>[4x]MKVAPAPASGQPGGGSKKPSDYGCQLHYKHARVVEPESTTDDGMKRLKDVGDKGTLITAAELGLVDKYRDLKRAGQDILTCDWPYHYSSILYACYGNQYKILQMVEREFVGSTQELTAMHTTRCWVGKNSAMVAAYQGHLETMLYIIDLDMQGKFTEDLFKQRDVMGKNAMMWAASQGHTDTIEVLLVRSLYRLLPEDCADPLVLKTRWKLVSLLADLASHCRDYDPGCSRSFFQEVLASIKYDPVEGARQEEAAAAGGGGSAREGAALHEPTWGVDDGEEEERRHGVKHSDLVGKSAASTTAAAAAGGKTASGKPGEPGGGGAVKLKDVHITVRTLQGVIVSAYRAGMNCMGVIMYCQSLLQQARYFDDLVAQLTAWEVKLLDTCRNKQEVQAILAPTEDDPSEPVGYALATFDKAFLSHKFVQQIFTEKWDTMGVTDYTKSLFGVVWGGCSLVVAFAAWATICPLVVVARSFLSPVQDFMMRGKVIVDSRFPWHVPLYRWLLTQCALITFTVLLSYLVFSFDPSDPVPASVAPLNTFLAVWCAAILVDEVQEYVEEGRAEYMSSGWNVMDVTMALSYILHYILRIIAVRVTDNLNILLVVNDLLAAAALMAWFRMVSVFELSSAIGPLIQMMKQMLIKDVTRFALLVLVILLGFSVGMEALFQEACIERDPTTNECTKYTSWGYDWQKDGLVGGMTFLQYIALGNANPVDFEQKRVTGVIFYLIFAIVTAILLLNLFIAMLADTYTRVSTQAMVEFRYRKAKLMASYSRRDFVCPPFNLLHLVCAAVGNGLRRLVWGPDGFTPVSMRKNETVPLFSWYFPQGEEMRQVVVLQRRVVDDFLNSNRVALFREKLNAELPNLVHEMLKQKGKGDGGALAGGGAAASTTVLATAVSVTAAAGH

Transient receptor potential (TRP) channels are ubiquitous cation-selective sensory ion channels that respond to numerous physical and chemical stimuli and are often considered polymodal signal integrators. In this study, we present cryo-electron microscopy (cryo-EM) structures of crTRP1. The crTRP1 architecture is unique; it exhibits overall C2 symmetry and its ankyrin repeat domain (ARD) appears to bend towards and interact with the lipid bilayer. In agreement with a previous study, we found that crTRP1 requires both heat and the lipid PIP2 for its activation.

We heterologously expressed the full-length crTRP1 in HEK 293S cells and purified it in the detergent glycol-diosgenin (GDN) or lauryl maltose neopentyl glycol (LMNG). The final reconstruction of crTRP1 in GDN exhibited an overall resolution of 3.53 Å, with higher resolution for the molecule’s core. For crTRP1 in GDN, the density for the P-loops was completely invisible, presumably due to their higher flexibility, while for crTRP1 in nanodisc, the purported helical portions of the P-loops were poorly resolved and modeled as poly-alanine helices. Regardless of its symmetry, the crTRP1 ion conduction pathway is occluded in both the GDN and nanodisc structures, as evidenced by a strong density in the middle of the ion channel pore. The hydrophobic environment at this narrow, gate-forming region of the pore suggests that the density may belong to a lipid. We identified twelve (three per subunit) well-resolved, non-protein densities in the crTRP1 cryo-EM map that are buried in the inter-subunit intramembrane interfaces. On the basis of the shapes of the putative lipid densities and the proximity of their apparent head domains to positively charged residues, we have modeled the site 1 and 2 densities as PIP2. The head of the site 3 putative lipid, which we modeled as phosphatidylcholine (PC), is surrounded by seven tyrosines, two from the pre-S1 elbow and five from the ARD fingers. Unlike structures of the majority of mammalian TRP channels, the rose-shaped structure of the crTRP1 homotetramer has twofold, rather than fourfold rotational symmetry. While deviation from the fourfold symmetry at the coiled coil region is accommodated by a simple swing of the coiled coil helices in subunits A/C relative to subunits B/D, the pore-forming S6 helices in B/D undergo one helical turn (~100°) rotation with respect to the S6 helices in A/C, exposing a different set of residues to the pore.> SYRHF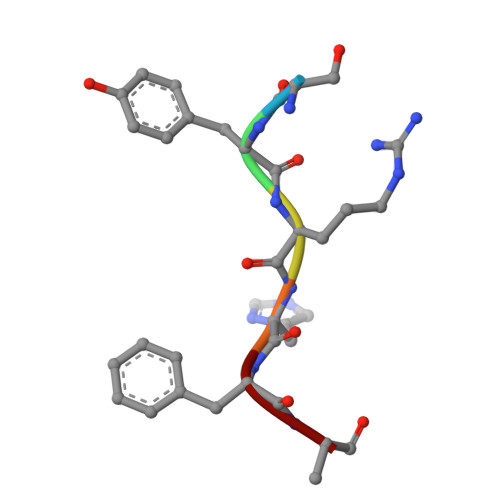A>MMFVRLSYH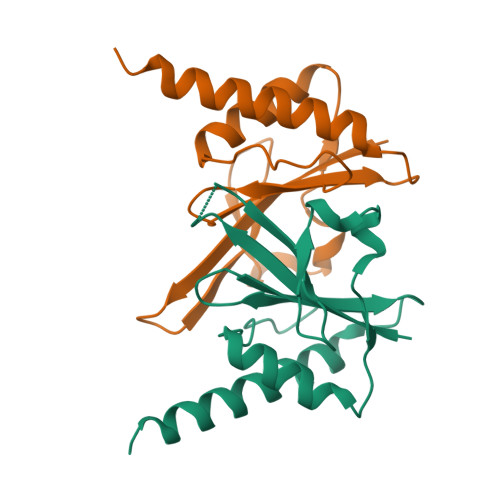SFDYLFNLFDAGVIDLNTKCPVSLSEIEDYDNFGWLELTAENLENVCEYCAKLGIEANGSLGDFRYWYSGDMSYHLELKSDQSENLEVKIREINLKLKELELIKNECLEHHHHHH[2x]> MNPIAVTLLTGFLGAGKTTLLR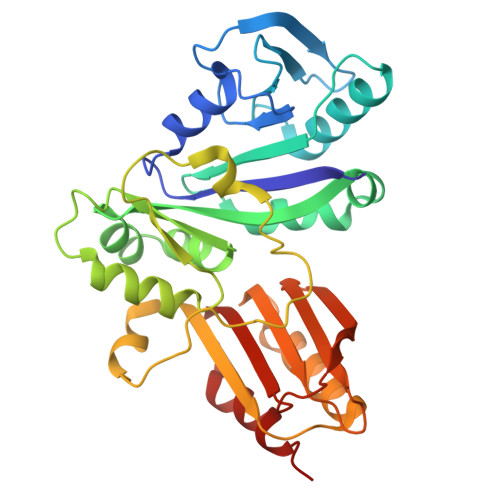HILNEQHGYKIAVIENEFGEVSVDDQLIGDRATQIKTLTNGCICCSRSNELEDALLDLLDNLDKGNIQFDRLVIECTGMADPGPIIQTFFSHEVLCQRYLLDGVIALVDAVHADEQMNQFTIAQSQVGYADRILLTKTDVAGEAEKLHERLARINARAPVYTVTHGDIDLGLLFNTNGFMLEENVVSTKPRFHFIADKQNDISSIVVELDYPVDISEVSRVMENLLLESADKLLRYKGMLWIDGEPNRLLFQGVQRLYSADWDRPWGDEKPHSTMVFIGIQLPEEEIRAAFAGLRK> CNIKNGRCEQFCKNSADNKVVCSCTEGYRLAENQKSCEPAVPFPCGRVSVSQT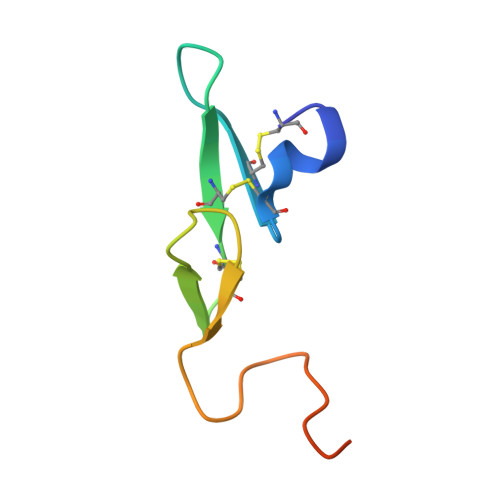SKLTR> MSKKQKKEITTTVTSEDHFMTFYNENNKKLIVVDVYPGWSGPCTAMYPTYNQLMISIDDFEKRIDILLLDQDKLVT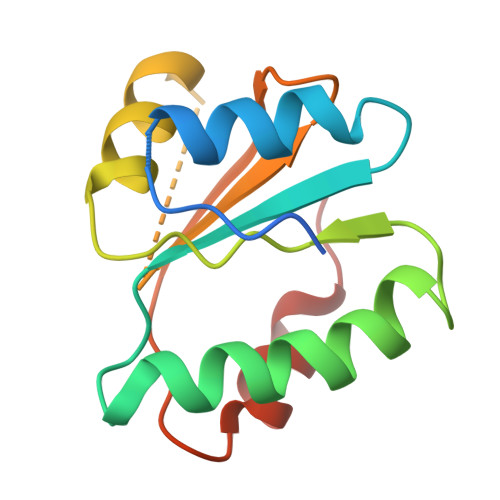YKNDKFHATCQPKFLFISEGKIIDEVLGTNIPVFIEKVNKYIPLSY(1~{S},3~{Z})-3-[(2~{E})-2-[(1~{S},3~{a}~{S},7~{a}~{S})-7~{a}-methyl-1-[(2~{S})-6-methyl-2-oxidanyl-heptan-2-yl]-2,3,3~{a},5,6,7-hexahydro-1~{H}-inden-4-ylidene]ethylidene]-4-methylidene-cyclohexan-1-ol 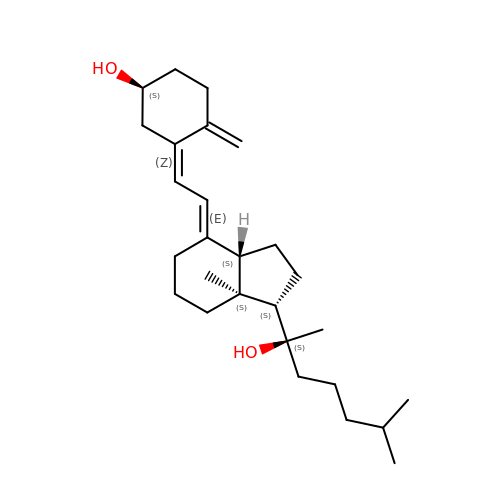| C27 H44 O2 | IQEQEOBGZMEDBQ-LBRHRNEPSA-N> GSTG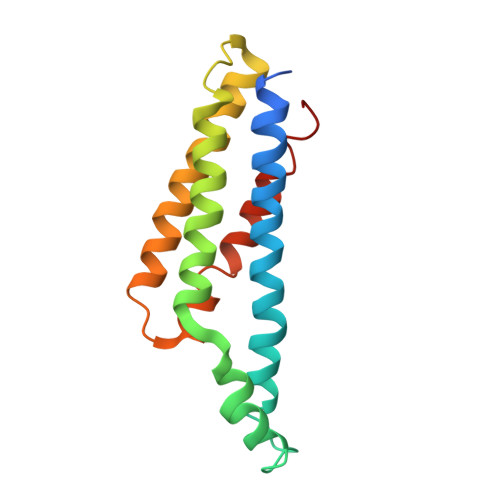SSNRYQSYLEGVKYNVDSAIQTITKIYNTYTLFSTKLTQMYSTRLDNFAKAKAKEEAAKFTKEDLEKNFKTLLNYIQVSVKTAANFVYINDTHAKRKLENIEAEIKTLIAKIKEQSNLYEAYKAIVTSILLMRDSLKEVQGIID> 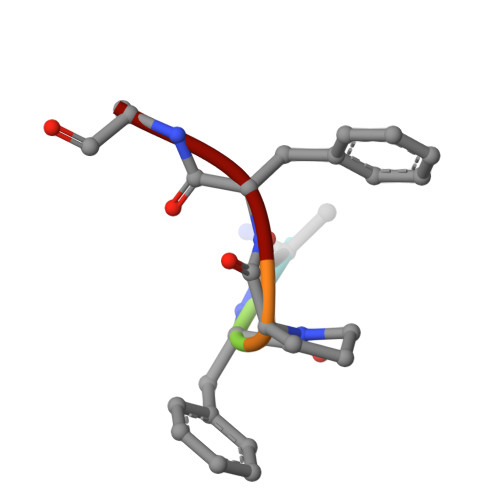QFPFV> ATTQIGEIVKTVANTVESEIKAELGVIPSLNAVETGATSNTEPEEAIQTRTVINMHGTAECLVENFLGRSALVCMRSFEYKNHSTSTSSIQKNFFIWTLNTRELVQIRRKMELFTYLRFDTEITIVPTLRLFSSSNVSFSGLPNLTLQAMYVPTGARKPSSQDSFEWQSACNPSVFFKINDPPARLTIPFMSINSAYANFYDGFAGFEKKATVLYGINPANTMGNLCLRVVNSYQPVQYTLTVRVYMKPKHIKAWAPRAPRTMPYTNILNNNYAGRSAAPNAPTAIVSHRSTIKTMPNDINLTTA;> SPSAEACGYSDRVLQLKLGNSSIVTQEAANICCAYGEWPTYLPDNEAVAIDKPTQPETSTDRFYTLKSKKWESNSTGWWWKLPDALNQIGMFGQNVQYHYLYRSGFLCHVQCNATKFHQGTLLIVAIPEHQIGKKGTGTSASFAEVMKGAEGGVFEQPYLLDDGTSLACALVYPHQWINLRTNNSATIVLPWMNSAPMDFALRHNNWTLAVIPVCPLAGGTGNTNTYVPITISIAPMCAEYNGLRNAITQ;> GVPTCLLPGSNQFLTTDDHSSAPAFPDFSPTPEMHIPGQVHSMLEIVQIESMMEINNVNDASGVERLRVQISAQSDMDQLLFNIPLDIQLEGPLRNTLLGNISRYYTHWSGSLEMTFMFCGSFMTTGKLIICYTPPGGSSPTDRMQAMLATHVVWDFG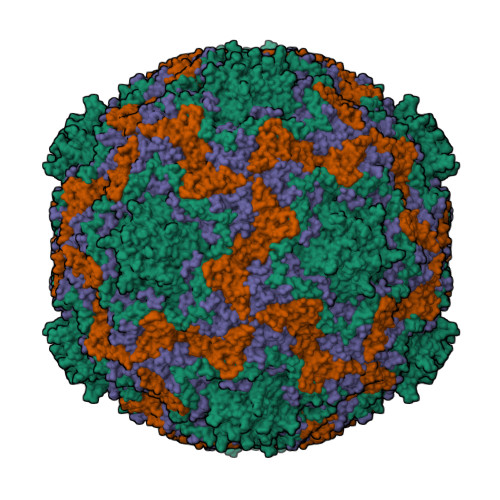LQSSITIIIPWISGSHYRMFNTDAKAINANVGYVTCFMQTNLVAPVGAADQCYIVGMVAAKKDFNLRLMRDSPDIGQSAILPEQA;> GAQVSRQQTGTHENANVATGGSSITYNQINFYKDSYAASASKQDFSQDPSKFTEPVAEALKAGAPVLK>[2x]MHHHHHHMNMLVDGEWRTDAHELTAGDGSFERQATTFRNWVQDDSDARFQPEAGRYHLYVSYACPWAHRTLVTRTLKGLEDAISVSVVDPYRAEDGWQFTPEKEGCTHDHVHDVDYLRELYVRAAPDVTCRVTVPVLWDTEEDTIVNNESEEIMRMFDTEFDEFADHTVDLYPEGYQEKVDQIIDNIYEPINNGVYRAGFATEQEPYDEAVAELFGALAHWDDVLADQRYLAGDRLTEADIAMF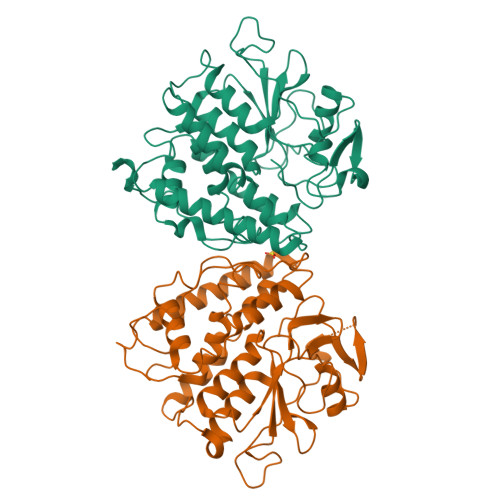TTLVRFDNVYHTHFMCNVQYIREFDNLWPYLRDLYQTHGIAETVEMDHITEHYYTTHPDVNPHRIVARGPDLDFEAPHSRDELAGEPPAALVSSAGR> GIDPFTSTQQHTEPAEEETLHNIITDTENVQGSFSKHEFQAETKKLLDIVARSLYSEKEVFIRELISNGSDALEKLRHRMITAGGDTAPMEIHLQTDSVKGTFTIQDTGVGMNKEDLVSNLGTIARSGSKAFLDALQNQAEASSSIIGQFGVGFYSAFMVADKVEVYSQSAEADAPGYKWSSDGSGVFEVAEASGVRQGTKIVLHLKDDCKEFSSEDRVKEVVTKYSNFVSFPIFLNGRRLNTLQALWMMEPKDISEWQHEEFYRYVAQAYDKPRYTLHYRADAPLNIRSIFYVPEMKPSMFDVSREMGSSVALYSRKILIQTKATDILPKWLRFLRGVVDSEDIPLNLSRELLQESALIRKLRDVLQQRVIRFLLDQSKKDPEKYARFFEDYGLFMREGIVTTGEQSVKEDIAKLLRFESSALPAGQQTSLMEYSSRMKAGTRNIYYLCAPNRHLAEHSPYFEAMKQKDMEVLFCFEQFDELTLLHLREFDRKKLISAETDIVVDHYKEEKFQDSKPASERLSSEQAEDLLAWMRNALVQRVTNIKVTPRLDTHPAMITVLEMGAARHFLRTQQLARSSEERAQILQPTLEINTGHDLIKKLHALKDSNPELAQLLLEQIYDNAMIAAGLNEDPRPMISRLNQLLTRALEKHGSDSATHIKFSKRDEDGKELAGATMELRDSSGKTISTWISDGQVKDFYLYPGKYTFVETAAPDGYEVATAITFTVNEQGQVTVNG;> GIDPFTSTQQHTEPAEEETLHNIITDTENVQGSFSKHEFQAETKKLLDIVARSLYSEKEVFIRELISNGSDALEKLRHRMITAGGDTAPMEIHLQTDSVKGTFTIQDTGVGMNKEDLVSNLGTIARSGSKAFLDALQNQAEASSSIIGQFGVGFYSAFMVADKVEVYSQSAEADAPGYKWSSDGSGVFEVAEASGVRQGTKIVLHLKDDCKEFSSEDRVKEVVTKYSNFVSFPIFLNGRRLNTLQALWMMEPKDISEWQHEEFYRYVAQAYDKPRYTLHYRADAPLNIRSIFYVPEMKPSMFDVSREMGSSVALYSRKILIQTKATDILPKWLRFLRGVVDSEDIPLNLSAELLQESALIRKLRDVLQQRVIRFLLDQSKKDPEKYARFFEDYGLFMREGIVTTGEQSVKEDIAKLLRFESSALPAGQQTSLMEYSSRMKAGTRNIYYLCAPNRHLAEHSPYFEAMKQKDMEVLFCFEQFDELTLLHLREFDRKKLISAETDIVVDHYKEEKFQDSKPASERLSSEQAEDLLAWMRNALVQRVTNIKVTPRLDTHPAMITVLEMGAARHFLRTQQLARSSEERAQILQPTLEINTGHDLIKKLHALKDSNPELAQLLLEQIYDNAMIAAGLNED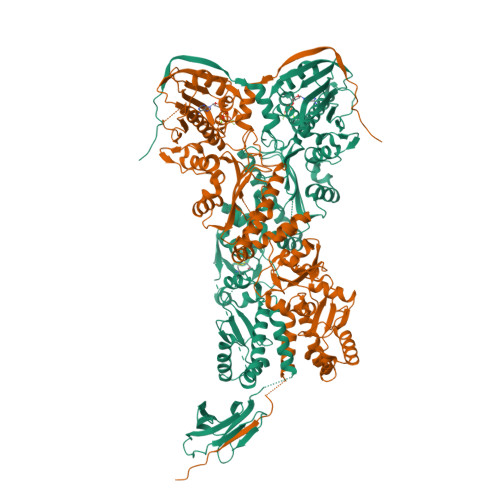PRPMISRLNQLLTRALEKHGGSGSSAHIVMVDAYKPTK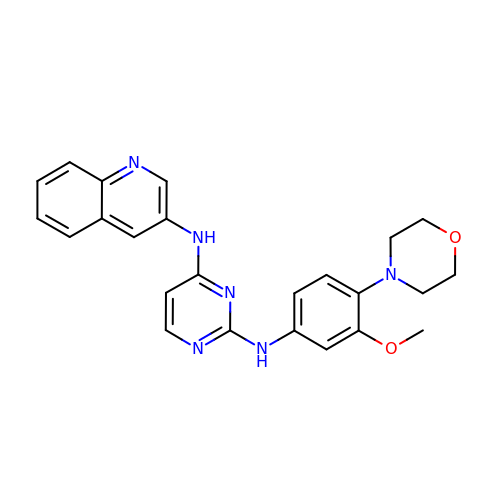N~2~-[3-methoxy-4-(morpholin-4-yl)phenyl]-N~4~-(quinolin-3-yl)pyrimidine-2,4-diamine | C24 H24 N6 O2 | LNEPMZDEABTAPY-UHFFFAOYSA-N>[5x]PVVIKTEGPAWTPLEPKLITRLADTVRTKGLRSPITMAEVEALMSSPLLPHDVTNLMRVILGPAPYALWMDAWGVQLQTVIAAATRDPRHPANGQGRGERTNLNRLKGLADGMVGNPQGQAALLRPGELVAITASALQAFREVARLAEPAGPWADIMQGPSESFVDFANRLIKAVEGSDLPPSARAPVIIDCFRQKSQPDIQQLIRTAPSTLTTPGEIIKYVLDRQKTA

As the virus buds from the cell, the viral protease cleaves Gag into several fragments, including the capsid protein (CA) that then assembles into the mature capsid shell (core), rendering the virus particle infectious. The CA portion of all retroviral Gag proteins folds into two separate domains, the N-terminal domain (CANTD) and C-terminal domain (CACTD). In mature lattices, CANTD interactions form only intra-hexamer and intra-pentamer interfaces, while CACTD interactions are also involved in formation of inter-hexamer and inter-pentamer interfaces. Our results show that, like lentiviruses, RSV is sensitive to IP6 in vitro and in cells, where in the mature CA lattice IP6 binds in a pore formed in the center of the CANTD hexamer.

To further understand how RSV CA is able to generate both regular tubular and pleomorphic polyhedral CLPs, and in particular how the different inter- and intra-hexameric CA interfaces allow for the observed flexibility, we also performed subtomogram averaging on polyhedral CLPs. Most important, we determined the structure of the mature CA pentamer in these polyhedrons to define the interactions between hexameric and pentameric RSV CA assembly states. Pentamers, on the other hand, organize rigid vertices, where the lattice is curved in different directions. The observation that within pleomorphic polyhedrons the CA pentamer constitutes the rigid building block prompted us to investigate if the pentamers within T = 1 icosahedrons and polyhedrons are structurally identical. We compared the model of T = 1 pentamers with the model of the pentamer derived from the polyhedrons. In fact, the two models are virtually superimposable, showing an RMSD of their C-alpha atoms of 0.74 Å. This finding further underscores the observations that the RSV CA pentamer (1) is very rigid due to the tighter packing of the CA domains in the pentamer, (2) always promotes the same local geometry, and (3) is independent in arrangement of the size and shape of the CLP. In contrast to the pliability of the RSV CA hexamer, the CA pentamer represents a rigid building block that acts as the local organization center that defines hexamer shape and, depending on the position on the lattice, overall core architecture.> MTAIVEAPQPGAEAIASPQAAVVAIMAADVQIAVVLDAHAPISVMIDPLLKVVNTRLRELGVAPLEAKGRGRWMLCLVDGTPLRPNLSLTEQEVYDGDRLWLKFLEDTEHRSEVIEHISTAVATNLSKR

The ESX-5 type VII secretion system is a membrane-spanning protein complex key to the virulence of mycobacterial pathogens. Key to their pathogenicity is the secretion of a wide range of virulence proteins via type VII secretion systems (T7SSs). The ESX-5 T7SS is found almost exclusively in slow growing, pathogenic mycobacteria and plays a key role in nutrient uptake and immune modulation during an infection. The importance of ESX-5 and other ESX secretion systems (ESX-1 to ESX-4) for the virulence of mycobacterial pathogens makes these membrane-spanning machineries a key target for the development of novel therapeutics.

The ubiquitin-like (Ubl) domains of EccD5 dimerize and interact with the cytoplasmic domain of EccE5 at the periphery of the ESX-5 complex. On the cytosolic side of the central pore, the EccD5 Ubl domain formed interactions with the EccC5 domain of unknown function (DUF), which follows the EccC5 stalk domain.> MAMKISVSKNDLENALRYLQAFLDKKDASSIASHIHLEVIKEKLFLKASDSDIGLKSYIFTQSSDKEGVGTINGKKFLDIISCLKDSNIILETKDDSLAIKQNKSSFKLPMFDADE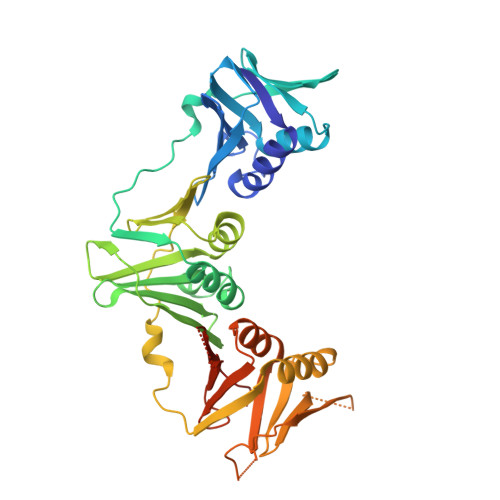FPEFPVIDPKVSIEVNAPFLVDAFKKIAPVIEQTSHKRELAGILMQFDQKHQTLSVVGTDTKRLSYTQLEKISIHSTEEDISCILPKRALLEILKLFYENFSFKSDGMLAVIENEMHTFFTKLIDGNYPDYQKILPKEYISSFTLGKEEFKESIKLCSSLSSTIKLTLEKNNALFESLDSEHSETAKTSVEIEKGLDIEKAFHLGVNAKFFLEALNALGTTQFVLRCNEPSSPFLIQESLDEKQSHLNAKISTLMMPITLELHHHHHH> GSHMASPNGQTKPLPALKLALEYIVPCMNKHGICVVDDFLGKETGQQIGDEVRALHDTGKFTDGQLVSQKSDSSKDIRGDKITWIEGKEPGCETIGLLMSSMDDLIRH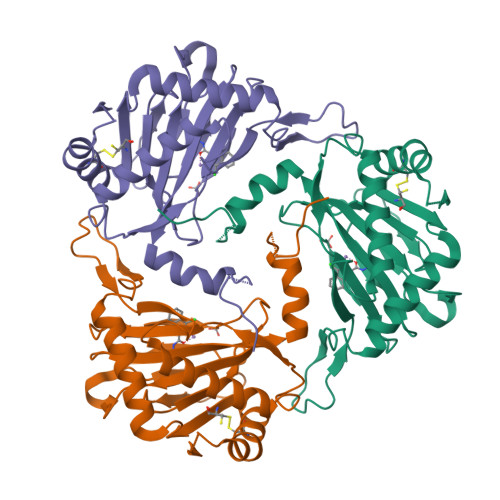CNGKLGSYKINGRTKAMVACYPGNGTGYVRHVDNPNGDGRCVTCIYYLNKDWDAKVSGGILRIFPEGKAQFADIEPKFDRLLFFWSDRRNPHEVQPAYATRYAITVWYFDADETARAKVKYLTGEKGVRVELNKPSDSVGKDVF> DPKKVLDKAKDQA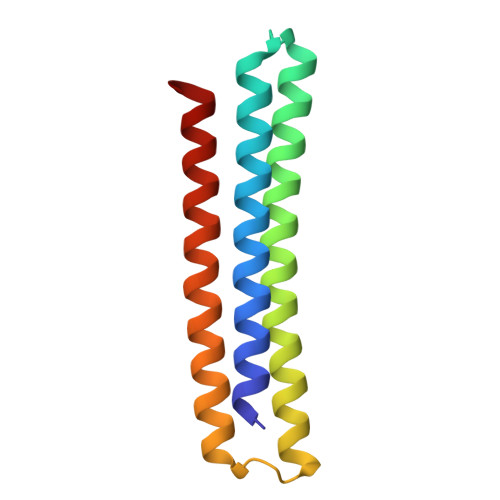ENRVRELKQVLEELYKEARKLDLTQEMRKKLIERYAAAIIRAIGDINNAIYQAKQEAEKLKKAGLVNSQQLDELLRRLDELQKEASRKANEYGREFELKLEYG> EQLTKCEVFRELKDLKGYGGVSLPEWVCTTFHTSGYDTQAIVQNNDSTEYGLFQINNKIWCKDDQNPHSSNICNISCDKFLDDDLTDDIMCVKKILDKVGINYWLAHKALCSEKLDQWLCEKL

In our study, we obtained bovine α-lactalbumin complexed with lanthanum ion (La3+-B-α-LA) and determined its high resolution crystal structure. The natural calcium binding site of bovine α-lactalbumin is replaced by lanthanum. The structure of the complex La3+-B-α-LA is composed of four α-helices and three antiparallel β-strands. The structure can be divided into α and β sub-domains and the presence of a cleft region clearly demarcates the existence of these two sub-domains.

The La3+ complex of apo-B-α-LA was crystallized as per the details given in the experimental section and the structure of the complex was established by single crystal X-ray diffraction at a resolution of 1.85 Å with one molecule in the asymmetric unit in P3121 space group. In the present structure, the La3+ is bound to the protein through the side chain carboxylate groups of Asp82, Asp87 and Asp88, and the main chain amide carbonyl groups of Lys79 and Asp84 in addition to three water molecules (W1, W2 and W3). In the structure of La3+-B-α-LA, the La3+ shows eight coordination with dodecahedral geometry while it is pentagonal bipyramidal w.r.t. Ca2+ in case of the Ca2+-B-α-LA structure. The analysis revealed that La3+ is coordinated in the metal binding cleft of B-α-LA with an additional water molecule as compared to that in the Ca2+ bound structure. The average La3+···O distance observed in the present structure (~2.5 Å) is longer than that observed for the average Ca2+···O distance (2.37 Å) by ~0.18 Å, supporting that the metal ion binding core expands in case of La3+ bound structure. Additionally, some unique conformational changes are observed for the amino acid side chains involved upon binding to La3+. The Asp82 and Asp87 side chains are in a similar plane for both the apo-B-α-LA and Ca2+-B-α-LA structures, while in La3+-B-α-LA, the side chain of Asp82 is rotated and hence the carboxylate group is almost perpendicular to what was observed in case of apo- and Ca2+ structures. The disulphide bond between Cys6-Cys120 in La3+-B-α-LA is flipped into an opposite orientation as compared to apo-B-α-LA and Ca2+-B-α-LA. A flexible loop (residues 105–110) below the cleft region adopts a helical conformation in La3+-B-α-LA complex. The average B factors suggest that the structure of the polypeptide in the La3+-B-α-LA complex is more rigid as compared to the other two structures.Phenylacetyl 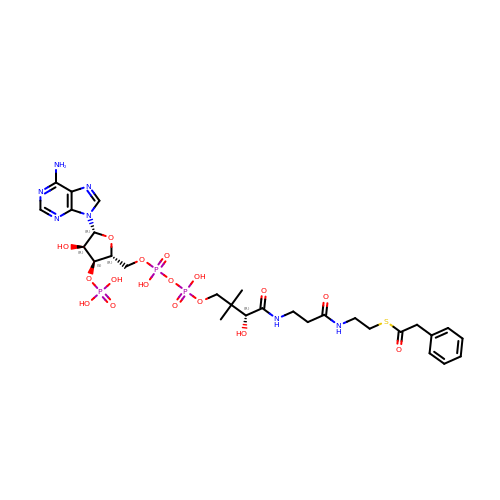coenzyme A | C29 H42 N7 O17 P3 S | ZIGIFDRJFZYEEQ-CECATXLMSA-N(~{E})-3-[2-[[2,6-bis(chloranyl)phenyl]methoxy]phenyl]-~{N}-oxidanyl-prop-2-enamide 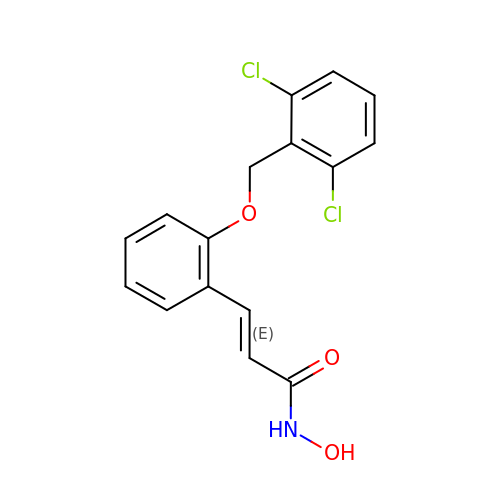| C16 H13 Cl2 N O3 | YTQRIEFQVODUBZ-CMDGGOBGSA-N N-tert-butyl-3-[(5-methyl-2-{[4-(4-methylpiperazin-1-yl)phenyl]amino}pyrimidin-4-yl)amino]benzenesulfonamide 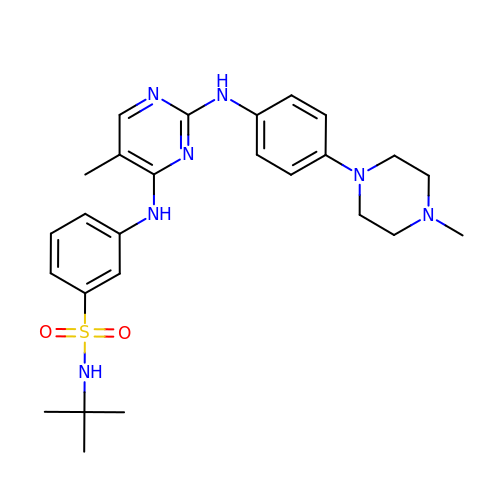| C26 H35 N7 O2 S | JVDOKQYTTYUYDV-UHFFFAOYSA-N>TPYDPLTLWTTPDPPPNCSLIQELDAKLTLCLTKNGSIVNGIVSLVGVKGNLLNIQSTTTTVGVHLVFDEQGRLITSTPTALVPQASWGYRQGQSVSTNTVTNGLGFMPNVSAYPRPNASEAKSQMVSLTYLQGDTSKPITMKVAFNGITSLNG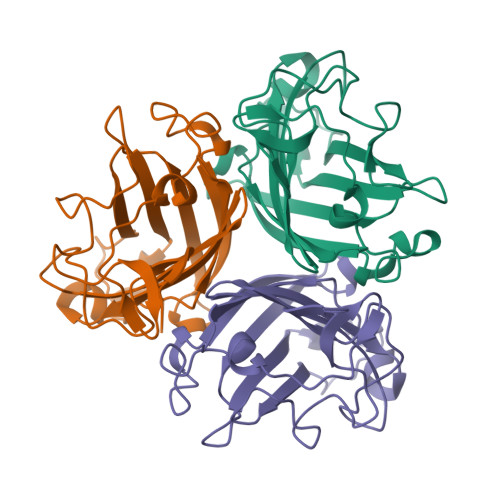YSLTFMWSGLSNYINQPFSTPSCSFSYITQE[6x]6-ethyl-4-methoxy-2-(pyridin-3-ylsulfanyl)-7H-pyrrolo[2,3-d]pyrimidine-5-carbaldehyde 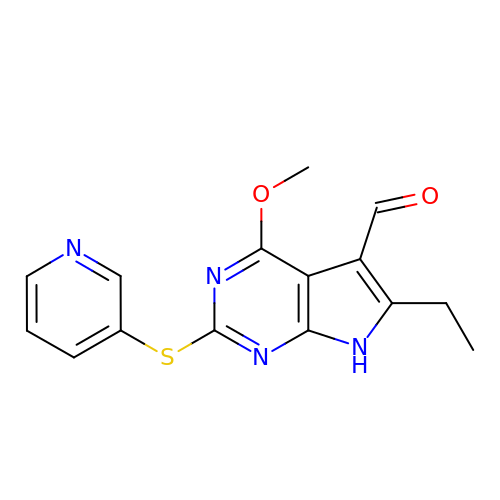| C15 H14 N4 O2 S | LEMXQPJEGCAOFY-UHFFFAOYSA-N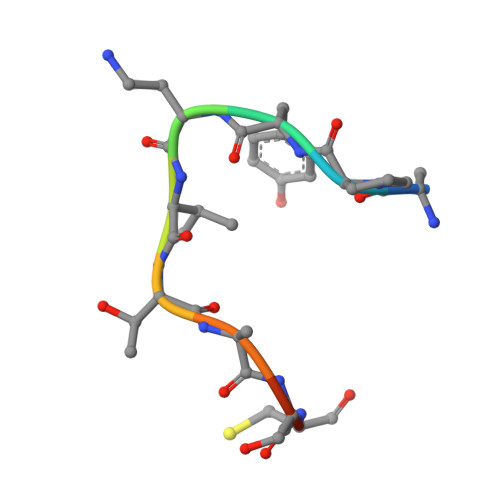> APYAVTASCR>MSKPKISLTKGKHPCTFCQARKVKCDRSLPACQNCIERNVTELCEYDDNGSRKRARLADDVNLYDKKLFNIWNQYERLWIHDTLGQCQQGVYMGIAFPLDVSEYNNTKDFYGYECLFSKESIFKILDHSLERLGWLYFGFFTDISELPYQMERYWNEYESMNINLENEEATTRQTTFKKSADQILWDLVLRSVIVMTIYYMPAKSILSLVDIDAIEKYPLDFSESNEGVDELKKKYEIFDYCLRHTLNKVLRTIFTLPPDVRTLQIFLILSNTNFLQIYPSLGNNILVHCIHLAKVLGIKDFKLKINDSGSTRLQKLSMHNIWFRLSTVDYMRSSPNKIIALHTDNSSALTRKTLFTHCSIDSIDVYDVESNLEVLRWKITSLDRDLEVSEPSLKTLKAMKELLGLLDRKTSVSNDASFNTKFESFFLKLQCNFVMWKILRYEFMQYGVTNGLQKLCCPARRIIALVANFLKEDYFEYTTHPFCVHILCVIAGFFSFYCIFHEADEVRDLRNDAVGLLKLLFDPLRPVISCFFSNLSRLEELRHIWKSVEITDQANRLVHPVMYVLKTDIIKLKRNLEIISGSLKDANYQETFKDKLEIDINTPALSSDFLEVVREFNLSHPLDINGKMSRQNN[2x];> MFDTKLFLSLPIDIRYTVYFFLGDVVQNVRPPAKSDIFNDELIAYPNIREFNQSLVDKYSKHIGVYDYIPNFIPNWCRDFDLLRHDIILTDRLRVCLQYEEQWFSVQWIVVSGELEIGIFTTDEQFLQVSYTINEYCHLLSIAQQDLRLGINVSDINDVNELCKEIQHRWLFDTVSYISFINCWDLDHENVVSIIPCMESFNNLHMLRIESKNMFNNLINTQGVRENPGKTIVYNVRQNIFELELYTLRDLGYKSVVDLQKWEQLQCLSLSGCEFIDLNNLILPQHCKMLILKEVKYIIWWDLSHLLKRIRPQWIINGQVKKPTKKEEEEESEWYNLYLEVVQTYQPLNFIELHNAKRVKGNLILPARLVTESRIKISNGTKVDSVLLI;> MSKENQNVVLVSVEGERFVVDRKIAERSLLLKNYLQDLNSGDLHDDNDADDDEDDEEDGDDEIVMPVPNVRSSVLQKVIEWAVHHKDSNFPDEDDDDSRKAAPVDP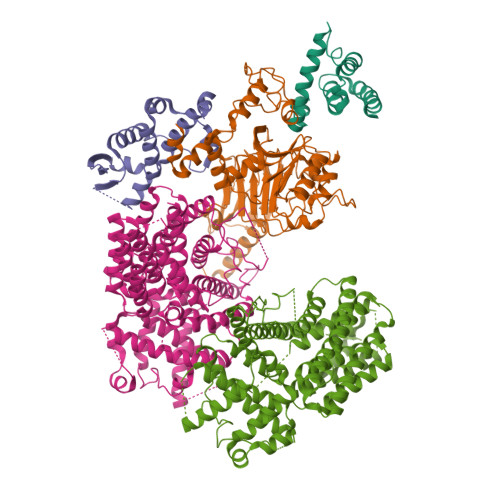WDREFLKVDQEMLYEIILAANYLNIKPLLDAGCKVVAEMIRGRTPEEIRRTFNIVNDFTPEEEAAIRRENEWAEDR;> MSKLDSLLKELPTRTAHLYRSIWHKYTEWLKTMPDLTGADLKLFLSQKYIVKYIASHDDIAKDPLPTCDAMIWFSRALDIENNDVLVLQQRLYGLVKLLEFDYSNVIAILQKISINLWNPSTDSLQSKHFKTCQDKLKLLLDFQWKFNTNVSFEDRTTVSLKDLQCILDDENGKCGLAHSSKPNFVLVPNFQSPFTCPIFTMAVYYYLRFHGVKKYYKGDGYQILSQLEHIPIIRGKSLDQYPRELTLGNWYPTIFKYCQLPYTKKHWFQVNQEWPQFPDFSDSSENTSTLAESDSENTIGIPDFYIEKMNRTKLQPCPQVHVHLFPTDLPPDIQAVFDLLNSVLVTSLPLLYRVFPTHDIFLDPSLKTPQNIAFLTGTLPLDIESQEHLLAQLIDKTGTVSEIGSG5-FLUOROURACIL | C4 H3 F N2 O2 | 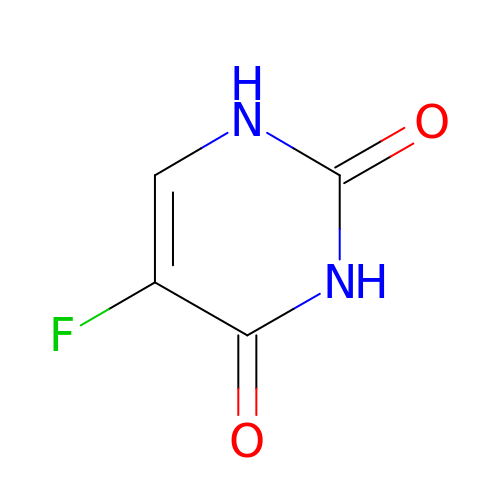GHASVSINZRGABV-UHFFFAOYSA-N> QKTRPFTVPNIPLKYLSNSRIPNPIEGMSLSPDQTQNVQFQNGRCTIDGQPLGTTPVSVSQLCKFRGRITSGQRVLNLTELDGSPFMAFAAPAPAGFPDLGSCDWHIEMSKIPNSSTQNNPIVTNSVKPNSQQFVPHLSSITLDENVSSGGDYIGTIQWTSPPSDSGGANTNFWKIPDYGSSLAEASQLAPAVYPPGFNEVIVYFMASIPGPNQSGSPNLVPCLLPQEYITHFISEQAPIQGEAALLHYVDPDTNRNLGEFKLYPGGYLTCVPNSSSTGPQQLPLDGVFVFASWVSRFYQLKPVGTAGPARGRL;>TRPFTVPNIPLKYLSNSRIPNPIEGMSLSPDQTQNVQFQNGRCTIDGQPLGTTPVSVSQLCKFRGRITSGQRVLNLTELDGSPFMAFAAPAPAGFPDLGSCDWHIEMSKIPNSSTQNNPIVTNSVKPNSQQFVPHLSSITLDENVSSGGDYIGTIQWTSPPSDSGGANTNFWKIPDYGSSLAEASQLAPAVYPPGFNEVIVYFMASIPGPNQSGSPNLVPCLLPQEYITHFISEQAPIQGEAALLHYVDPDTNRNLGEFKLYPGGYLTCVPNSSSTGPQQLPLDGVFVFASWVSRFYQLKPVG[2x];> TRPFTVPNIPLKYLSNSRIPNPIEGMSLSPDQTQNVQFQNGRCTIDGQPLGTTPVSVSQLCKFRGRITSGQRVLNLTELDGSPFMAFAAPAPAGFPDLGSCDWHIEMSKIPNSSTQNNPIVTNSVKPNSQQFVPHLSSITLDENVSSGGDYIGTIQWTSPPSDSGGANTNFWKIPDYGSSLAEASQLAPAVYPPGFNE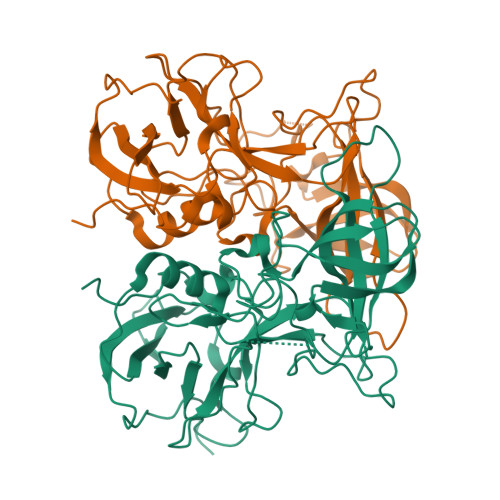VIVYFMASIPGPNQSGSPNLVPCLLPQEYITHFISEQAPIQGEAALLHYVDPDTNRNLGEFKLYPGGYLTCVPNSSSTGPQQLPLDGVFVFASWVSRFYQLKPVGTAGPA> MKMRTEKQIYDTILNFAKADDRIRVVTLEGSRTNINIIPDDFQDYDITFF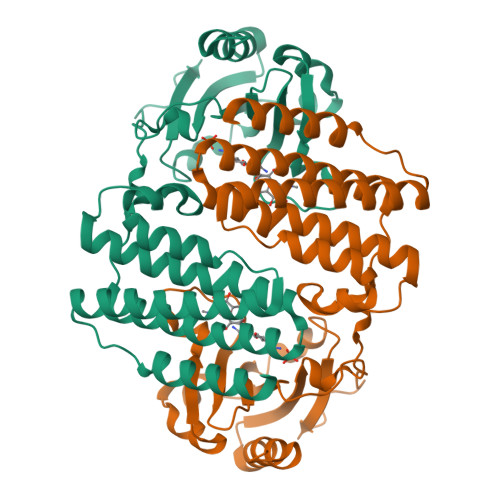VTDMQSFINSDEWLNVFGERLIMQKPEDMELFPKEEKGYSYLMLFWDGVKIDLTLLPLEVLDEYFTWDKLVKLLLDKDNRVTNIPVPTDEDYYIEHPTARSFDDCCNEFWNTVTYVVKGLCRKEILFAIDHLNNIVRMELLRMISWKVGIEQGYSFSLGKNYKFLERYISPELWKKILATYNMGSYTEMWKSLELCMGIFRMVSKEVAQCLNYLYPDYDKNISNYVIRQKEKYQRDPNSSSVDKLAAALEHHHHHH> SSELFTLTYGALVTQLCKDYENDEDVNKQLDRMGYNIGVRLI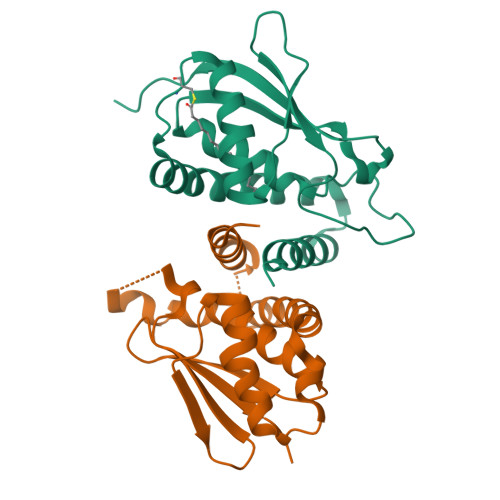EDFLARSNVGRCHDFRETADVIAKVAFKMYLGITPSITNWSPAGDEFSLILENNPLVDFVELPDNHSALIYSNLLCGVLRGALEMVQMAVEAKFVQDTLKGDGVTEIRMRFIRRIEDNL;> GMADTVLFEFLHTEMVAELWAHDPDPGPGGQKMSLSVLEGMGFRVGQALGERLPRETLAFREELDVLKFLCKDLWVAVFQKQMDSLRTNHQGTYVLQDNSFPLLLPMASGLQYLEEAPKFLAFTCGLLRGALYTLGIESVVTASVAALPVCKFQVVIPKS> MEEQPQMQDADEPADSGGEGRAGGPPQVAGAQAACSEDRMTLLLRLRAQTKQQLLEYKSMVDASEEKTPEQIMQEKQIEAKIEDLENEIEEVKVAFEIKKLALDRMRLSTALKKNLEKISRQSSVLMDNMKHLLELNKLIMKSQQESWDLEEKLLDIRKKRLQLKQASESKLLEIQTEKNKQKIDLDSMENSERIKIIRQNLQMEIKITTVIQHVFQNLILGSKVNWAEDPALKEIVLQLEKNVDMM;> MSPQKRVKNVQAQNRTSQGSSSFQTTLSAWKVKQDPSNSKNISKHGQNNPVGDYEHADDQAEEDALQMAVGYFEKGPIKASQNKDKTLEKHLKTVENVAWKNGLASEEIDILLNIALSGKFGNAVNTRILKCMIPATVISEDSVVKAVSWLCVGKCSGSTKVLFYRWLVAMFDFIDRKEQINLLYGFFFASLQDDALCPYVCHLLYLLTKKENVKPFRVRKLLDLQAKMGMQPHLQALLSLYKFFAPALISVSLPVRKKIYFKNSENLWKTALLAVKQRNRGPSPEPLKLMLGPANVRPLKRKWNSLSVIPVLNSSSYTKECGKKEMSLSDCLNRSGSFPLEQLQSFPQLLQNIHCLELPSQMGSVLNNSLLLHYINCVRDEPVLLRFYYWLSQTLQEECIWYKVNNYEHGKEFTNFLDTIIRAECFLQEGFYSCEAFLYKSLPLWDGLCCRSQFLQLVSWIPFSSFSEVKPLLFDHLAQLFFTSTIYFKCSVLQSLKELLQNWLLWLSMDIHMKPVTNSPLETTLGGSMNSVSKLIHYVGWLSTTAMRLESNNTFLLHFILDFYEKVCDIYINYNLPLVVLFPPGIFYSALLSLDTSILNQLCFIMHRYRKNLTAAKKNELVQKTKSEFNFSSKTYQEFNHYLTSMVGCLWTSKPFGKGIYIDPEILEKTGVAEYKNSLNVVHHPSFLSYAVSFLLQESPEERTVNVSSIRGKKWSWYLDYLFSQGLQGLKLFIRSSVHHSSIPRAEGINCNNQY;> MNQEDLDPDSTTDVGDVTNTEEELIRECEEMWKDMEECQNKLSLIGTETLTDSNAQLSLLIMQVKCLTAELSQWQKKTPETIPLTEDVLITLGKEEFQKLRQDLEMVLSTKESKNEKLKEDLEREQRWLDEQQQIMESLNVLHSELKNKVETFSESRIFNELKTKMLNIKEYKEKLLSTLGEFLEDHFPLPDRSVKKKKKNIQESSVNLITLHEMLEILINRLFDVPHDPYVKISDSFWPPYVELLLRNGIALRHPEDPTRIRLEAFHQ;> MDSYSAPESTPSASSRPEDYFIGATPLQKRLESVRKQSSFILTPPRRKIPQCSQLQEDVDPQKVAFLLHKQWTLYSLTPLYKFSYSNLKEYSRLLNAFIVAEKQKGLAVEVGEDFNIKVIFSTLLGMKGTQRDPEAFL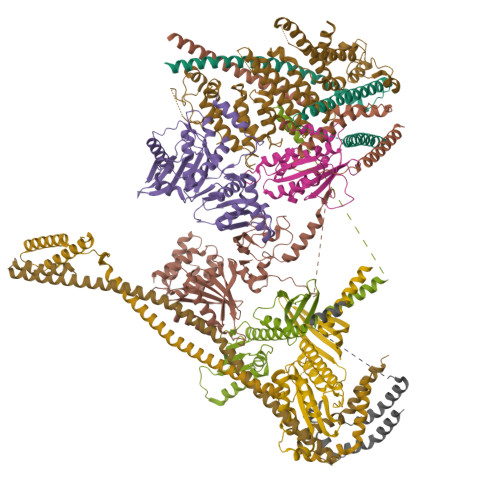VQIVSKSQLPSENREGKVLWTGWFCCVFGDSLLETVSEDFTCLPLFLANGAESNTAIIGTWFQKTFDCYFSPLAINAFNLSWMAAMWTACKMDHYVATTEFLWSVPCSPQSLDISFAIHPEDAKALWDSVHKTPGEVTQEEVDLFMDCLYSHFHRHFKIHLSATRLVRVSTSVASAHTDGKIKILCHKYLIGVLAYLTELAIFQIE;> MSVLRPLDKLPGLNTATILLVGTEDALLQQLADSMLKEDCASELKVHLAKSLPLPSSVNRPRIDLIVFVVNLHSKYSLQNTEESLRHVDASFFLGKVCFLATGAGRESHCSIHRHTVVKLAHTYQSPLLYCDLEVEGFRATMAQRLVRVLQICAGHVPGVSALNLLSLLRSSEGPSLEDL;> MDETVAEFIKRTILKIPMNELTTILKAWDFLSENQLQTVNFRQRKESVVQHLIHLCEEKRASISDAALLDIIYMQFHQHQKVWEVFQMSKGPGEDVDLFDMKQFKNSFKKILQRALKNVTVSFRETEENAVWIRIAWGTQYTKPNQYKPTYVVYYSQTPYAFTSSSMLRRNTPLLGQALTIASKHHQIVKMDLRSRYLDSLKAIVFKQYNQTFETHNSTTPLQERSLGLDINMDSRIIHENIVEKERVQRITQETFGDYPQPQLEFAQYKLETKFKSGLNGSILAEREEPLRCLIKFSSPHLLEALKSLAPAGIADAPLSPLLTCIPNKRMNYFKIRDK;> MEQANPLRPDGESKGGVLAHLERLETQVSRSRKQSEELQSVQAQEGALGTKIHKLRRLRDELRAVVRHRRASVKACIANVEPNQTVEINEQEALEEKLENVKAILQAYHFTGLSGKLTSRGVCVCISTAFEGNLLDSYFVDLVIQKPLRIHHHSVPVFIPLEEIAAKYLQTNIQHFLFSLCEYLNAYSGRKYQADRLQSDFAALLTGPLQRNPLCNLLSFTYKLDPGGQSFPFCARLLYKDLTATLPTDVTVTCQGVEVLSTSWEEQRASHETLFCTKPLHQVFASFTRKGEKLDMSLVS;> MDAELAEVRALQAEIAALRRACEDPPAPWEEKSRVQKSFQAIHQFNLEGWKSSKDLKNQLGHLESELSFLSTLTGINIRNHSKQTEDLTSTEMTEKSIRKVLQRHRLSGNCHMVTFQLEFQILEIQNKERLSSAVTDLNIIMEPTECSELSEFVSRAEERKDLFMFFRSLHFFVEWFEYRKRTFKHLKEKYPDAVYLSEGPSSCSMGIRSASRPGFELVIVWRIQIDEDGKVFPKLDLLTKVPQRALELDKNRAIETAPLSFRTLVGLLGIEAALESLIKSLCAEENN;> MSGKANASKKNAQQLKRNPKRKKDNEEVVLSENKVRNTVKKNKNHLKDLSSEGQTKHTNLKHGKTAASKRKTWQPLSKSTRDHLQTMMESVIMTILSNSIKEKEEIQYHLNFLKKRLLQQCETLKVPPKKMEDLTNVSSLLNMERARDKANEEGLALLQEEIDKMVETTELMTGNIQSLKNKIQILASEVEEEEERVKQMHQINSSGVLSLPELSQKTLKAPTLQKEILALIPNQNALLKDLDILHNSSQMKSMSTFIEEAYKKLDAS;> MPVKRSLKLDGLLEENSFDPSKITRKKSVITYSPTTGTCQMSLFASPTSSEEQKHRNGLSNEKRKKLNHPSLTESKESTTKDNDEFMMLLSKVEKLSEEIMEIMQNLSSIQALEGSRELENLIGISCASHFLKREMQKTKELMTKVNKQKLFEKSTGLPHKASRHLDSYEFLKAILN;> MAPRGRRRPRPHRSEGARRSKNTLERTHSMKDKAGQKCKPIDVFDFPDNSDVSSIGRLGENEKDEETYETFDPPLHSTAIYADEEEFSKHCGLSLSSTPPGKEAKRSSDTSGNEASEIESVKISAKKPGRKLRPISDDSESIEESDTRRKVKSAEKISTQRHEVIRTTASSELSEKPAESVTSKKTGPLSAQPSVEKENLAIESQSKTQKKGKISHDKRKKSRSKAIGSDTSDIVHIWCPEGMKTSDIKELNIVLPEFEKTHLEHQQRIESKVCKAAIATFYVNVKEQFIKMLKESQMLTNLKRKNAKMISDIEKKRQRMIEVQDELLRLEPQLKQLQTKYDELKERKSSLRNAAYFLSNLKQLYQDYSDVQAQEPNVKETYDSSSLPALLFKARTLLGAESHLRNINHQLEKLLDQG> MRVLILGVNGFIGNHLTERLLREDHYEVYGLDIGSDAISRFLNHPHFHFVEGDISIHSEWIEYHVKKCDVVLPLVAIATPIEYTRNPLRVFELDFEENLRIIRYCVKYRKRIIFPSTSEVYGMCSDKYFDEDHSNLIVGPVNKPRWIYSVSKQLLDRVIWAYGEKEGLQFTLFRPFNWMGPRLDNLNAARIGSSRAITQLILNLVEGSPIKLIDGGKQKRCFTDIRDGIEALYRIIENAGNRCDGEIINIGNPENEASIEELGEMLLASFEKHPLRHHFPPFAGFRVV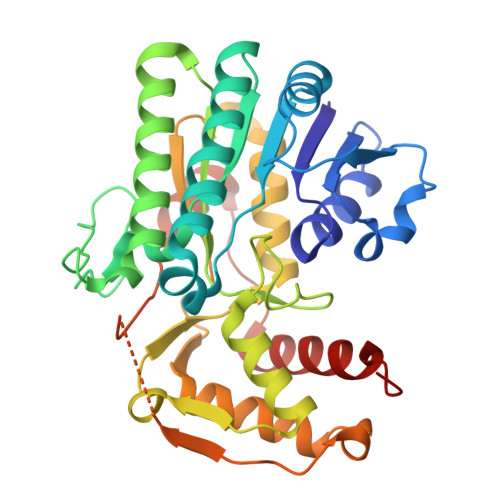ESSSYYGKGYQDVEHRKPSIRNAHRCLDWEPKIDMQETIDETLDFFLRTVDLTDKPS> MAHHHHHHEFPKPEFMSKSLEELQIGTYANIAMVRTTTPVYVALGIFVQHRVSALPVVDEKGRVVDIYSKFDVINLAAEK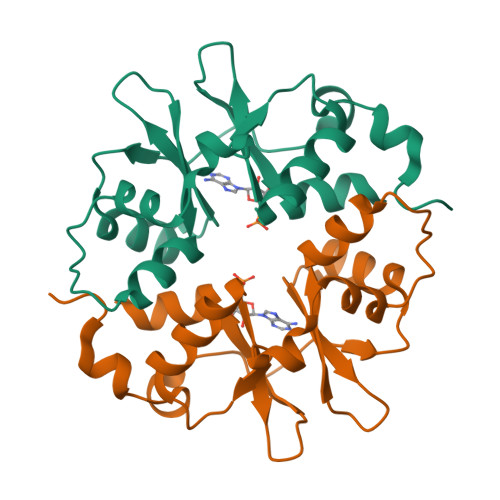TYNNLDVSVTKALQHRSHYFEGVLKCYLHETLETIINRLVEAEVHQLVVVDENDVVKGIVSLSDILQALVLT> GLIVDTRDVEERVHVMRKTKLAPTVAHGVFNPEFGPAALSNKDPRLNEGVVLDEVIFSKHKGDTKMSAEDKALFRRCAADYASRLHSVLGTANAPLSIYEAIKGVDGLDAMEPDTAPGLPWAL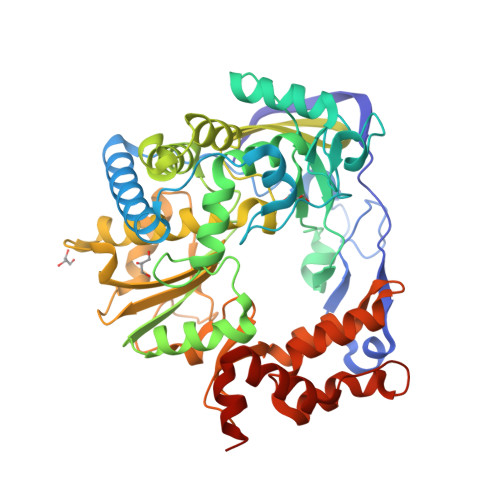QGKRRGALIDFENGTVGPEVEAALKLMEKREYKFACQTFLKDEIRPMEKVRAGKTRIVDVLPVEHILYTRMMIGRFCAQMHSNNGPQIGSAVGCNPDVDWQRFGTHFAQYRNVWDVDYSAFDANHCSDAMNIMFEEVFRTEFGFHPNAEWILKTLVNTEHAYENKRITVEGGMPSGCSATSIINTILNNIYVLYALRRHYEGVELDTYTMISYGDDIVVASDYDLDFEALKPHFKSLGQTITPADKSDKGFVLGHSITDVTFLKRHFHMDYGTGFYKPVMASKTLEAILSFARRGTIQEKLISVAGLAVHSGPDEYRRLFEPFQGLFEIPSYRSLYLRWVNAVCGDAAAALEHHHHHH>PVTKTRLIDTPVRSGQRIYAPQCDLIVTSHVSAGAELIADGNIHVYGMMRGRALAGASGDRETQIFCTNLMAELVSIAG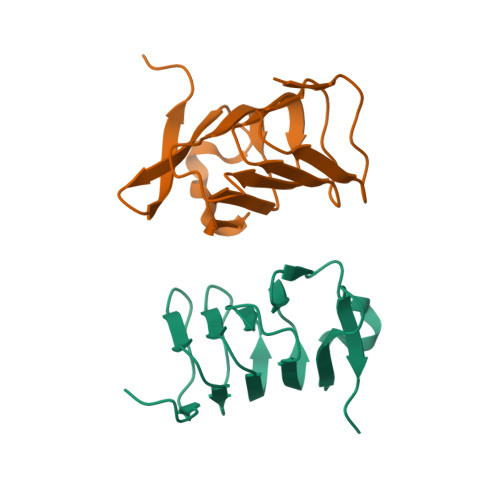EYWLSDQIPAEFYGKAARLQLVENALTVQPLNLEHHHHHH[2x]>MGNDISLIALLAFSTLLPFIIASGTCFVKFSIVFVMVRNALGLQQIPSNMTLNGVALLLSMFVMWPIMHDAYVYFEDEDVTFNDISSLSKHVDEGLDGYRDYLIKYSDRELVQFFENAQLKRQYGEETETVKRDKDEIEKPSIFALLPAYALSEIKSAFKIGFYLYLPFVVVDLVVSSVLLALGMMMMSPVTISTPIKLVLFVALDGWTLLSKGLILQYMDIAT[5x];> MFYALYFEIHHLVASAALGFARVAPIFFFLPFLNSGVLSGAPRNAIIILVALGVWPHALNEAPPFLSVAMIPLVLQEAAVGVMLGCLLSWPFWVMHALGCIIDNQRGATLSSSIDPANGIDTSEMANFLNMFAAVVYLQNGGLVTMVDVLNKSYQLCDPMNECTPSLPPLLTFINQVAQNALVLASPVVLVLLLSEVFLGLLSRFAPQMNAFAISLTVKSGIAVLIMLLYFSPVLPDNVLRLSFQATGLSSWFYERGATHVLE;>[4x]MDDLVFAGNKALYLVLILSGWPTIVATIIGLLVGLFQTVTQLQEQTLPFGIKLLGVCLCLFLLSGWYGEVLLSYGRQVIFLALAKG;>[16x]MKTHILLARVLACAALVLVTPGYSSEKIPVTGSGFVAKDDSLRTFFDAMALQLKEPVIVSKMAARKKITGNFEFHDPNALLEKLSLQLGLIWYFDGQAIYIYDASEMRNAVVSLRNVSLNEFNNFLKRSGLYNKNYPLRGDNRKGTFYVSGPPVYVDMVVNAATMMDKQNDGIELGRQKIGVMRLNNTFVGDRTYNLRDQKMVIPGIATAIERLLQGEEQPLGNIVSSEPPAMPAFSANGEKGKAANYAGGMSLQEALKQNAAAGNIKIVAYPDTNSLLVKGTAEQVHFIEMLVKALDVAKRHVELSLWIVDLNKSDLERLGTSWSGSITIGDKLGVSLNQSSISTLDGSRFIAAVNALEEKKQATVVSRPVLLTQENVPAIFDNNRTFYTKLIGERNVALEHVTYGTMIRVLPRFSADGQIEMSLDIEDGNDKTPQSDTTTSVDALPEVGRTLISTIARVPHGKSLLVGGYTRDANTDTVQSIPFLGKLPLIGSLFRYSSKNKSNVVRVFMIEPKEIVDPLTPDASESVNNILKQSGAWSGDDKLQKWVRVYLDRGQEAIK;>[6x]MSIATIVPENAVIGQAVNIRSMETDIVSLDDRLLQAFSGSAIATAVDKQTITNRIEDPNLVTDPKELAISQEMISDYNLYVSMVSTLTRKGVGAVETLLRS;>[13x]MATPWSGYLDDVSAKFDTGVDNLQTQVTEALDKLAAKPSDPALLAAYQSKLSEYNLYRNAQSNTVKVFKDIDAAIIQNFR;>METSKEKTITSPGPYIVRLLNSSLNGCEFPLLTGRTLFVVGQSDALTASGQLPDIPADSFFIPLDHGGVNFEIQVDTDATEIILHELKEGNSESRSVQLNTPIQVGELLILIRPESEPWVPEQPEKLETSAKKNEPRFKNGIVAALAGFFILGIGTVGTLWILNSPQRQAAELDSLLGQEKERFQVLPGRDKMLYVAAQNERDTLWARQVLARGDYDKNARVINENEENKRISIWLDTYYPQLAYYRIHFDEPRKPVFWLSRQRNTMSKKELEVLSQKLRALMPYADSVNITLMDDVTAA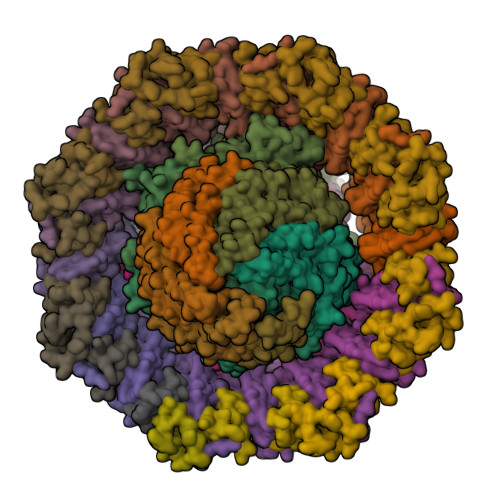GQAEAGLKQQALPYSRRNHKGGVTFVIQGALDDVEILRARQFVDSYYRTWGGRYVQFAIELKDDWLKGRSFQYGAEGYIKMSPGHWYFPSPL[24x]> ISGGDAIYSSTGRCSLGFNVRSGSTYYFLTAGHCTDGATTWWANSARTTVLGTTSGSSFPNNDYGIVRYTNTTIPKDGTVGGQDITSAANATVGMAVTRRGSTTGTHSGSVTALNATVNYGGGDVVYGMIRTNVCAEPGDSGGPLYSGTRAIGLTSGGSGNCSSGGTTFFQPVTEALVAYGVSVY;> VDCSEYPKPACTGEYR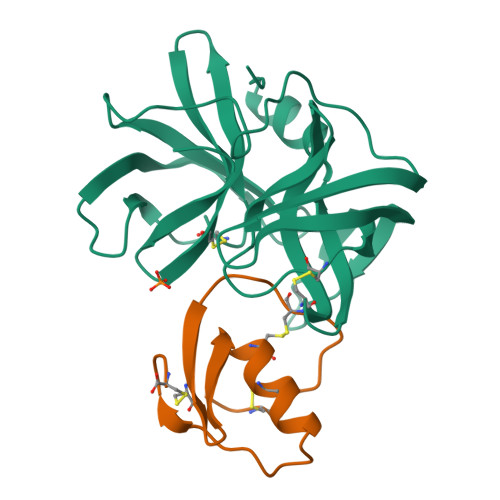PLCGSDNKTYGNKCNFCNAVVESNGTLTLSHFGKC>MEQCGAQAGGARCPNCLCCSRWGWCGTTSDFCGDGCQSQCSGCGPTPTPTPPSPSDGVGSIVPRDLFERLLLHRNDGACPARGFYTYEAFLAAAAAFPAFGGTGNTETRKREVAAFLGQTSHETTGGWPTAPDGPFSWGYCFKQEQNPPSDYCQPSPEWPCAP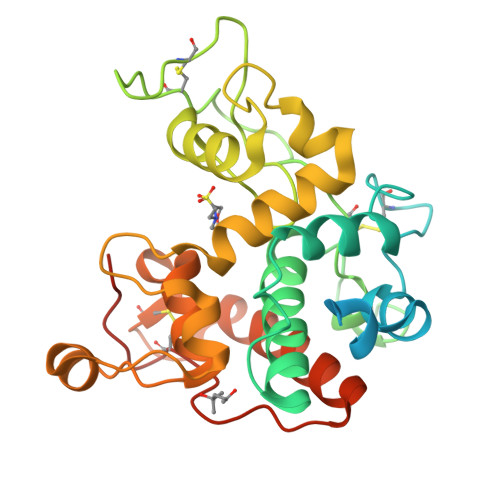GRKYYGRGPIQLSFNFNYGPAGRAIGVDLLSNPDLVATDATVSFKTALWFWMTPQGNKPSSHDVITGRWAPSPADAAAGRAPGYGVITNIVNGGLECGHGPDDRVANRIGFYQRYCGAFGIGTGGNLDCYNQRPFNSGSSVGLAEQ[2x]> GPGQKECDNALRQLETVRELLENPVQPINDMSYFGCLDSVMENSKVLGEAMTGISQNAKNGNLPEFGDAIATASKALCGFTEAAAQAAYLVGVSDPNSQAGQQGLVEPTQFARANQAIQMACQSLGEPGCTQAQVLSAATIVAKHTSALCNSCRLASARTANPTAKRQ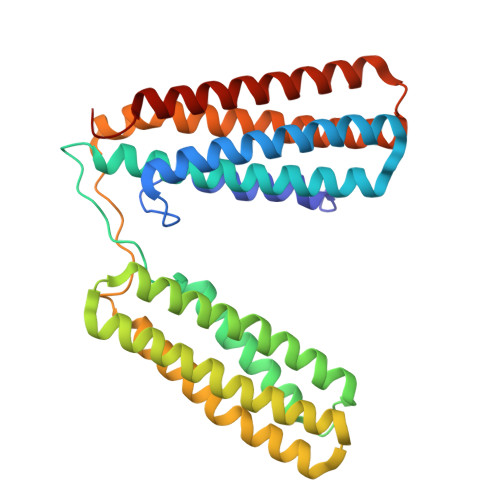FVQSAKEVANSTANLVKTIKALDGDFTEENRAQCRAATAPLLEAVDNLSAFASNPEFSSVPAQISPEGRAAMEPIVISAKTMLESAGGLIQTARALAVNPRDPPRWSVLAGHSRTVSDSIKKLITSMRDKAPGQL> GGGA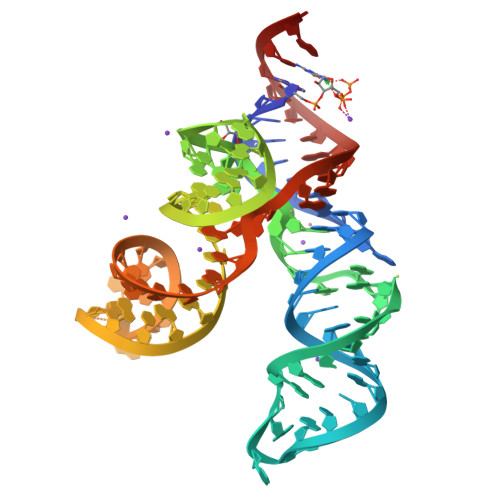ACUGAGCAGGCAAUGACCAGAGCGGUCAUGCAGCCGGGCUGCGAAAGCGGCAACAGAUGAUUACACGCACAUCUGUGGGACAGUUCCCAC> ATAAEIAALPRQKVELVDPPFVHAHSQVAEGGPKVVEFTMVIEEKKIVIDDAGTEVHAMAFNGTVPGPLMVVHQDDYLELTLINPETNTLMHNIDFHAATGALGGGGLTEINPGEKTILRFKATKPGVFVYHCAPPGMVPWHVVSGLNGAIMVLPREGLHDGKGKALTYDKIYYVGEQDFYVPRDENGKYKKYEAPGDAYEDTV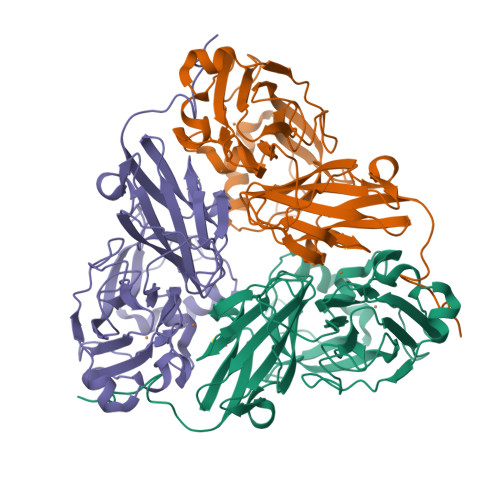KVMRTLTPTHVVFNGAVGALTGDKAMTAAVGEKVLIVHSQANRDTRPHLIGGHGDYVWATGKFNTPPDVDQETWFIPGGAAGAAFYTFQQPGIYAYVNHNLIEACELGAAAHFKVTGEWNDDLMTSVLAPSG>MTKVDFWPTLKDAYEPLYPQQLEILRQQVVSEGGPTATIQSRFNYAWGLIKSTDVNDERLGVKILTDIYKEAESRRRECLYYLTIGCYKLGEYSMAKRYVDTLFEHERNNKQVGALKSMVEDKIQKETL[2x];>GSHMQKGQVGIFSFQNNYADSATTFRILAHLDEQRYPLPNGAAEKNLPSL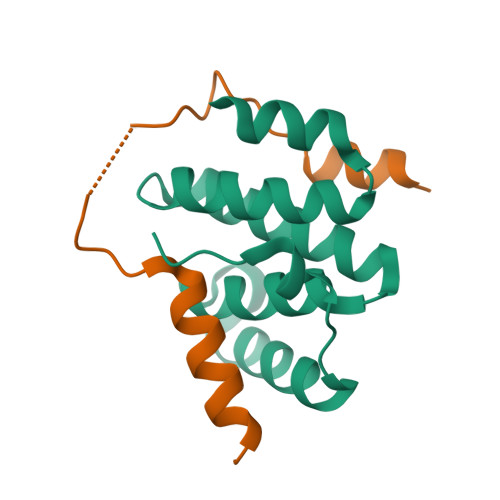FEGFKATVSIIQQR[2x]N-methyl-1-[3-(morpholin-4-ylmethyl)phenyl]methanamine | C13 H20 N2 O | 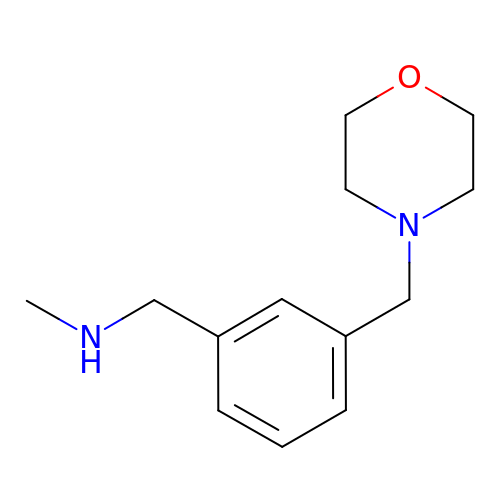JZMYRFZAMCXUIF-UHFFFAOYSA-N>MEQAAPRVVAFLSDVGTHDEATGLCKGLMSRICPGVTIIDITHQVPAFDVVEGALMLEDVPEFFPEHTVICAYVYPETGSGTPTVAVRNDKGQLLVAPDNGLLTRALDASGVAEARLVTNPAVMNHPPTPTWYGRDVVAACAAHLAAGTPLADVGPVVDDPVRLPDVPFTRHESGLVGRVARIDRAFGNVWTNIPSAALGLPSTPDGPVTLDATVGGE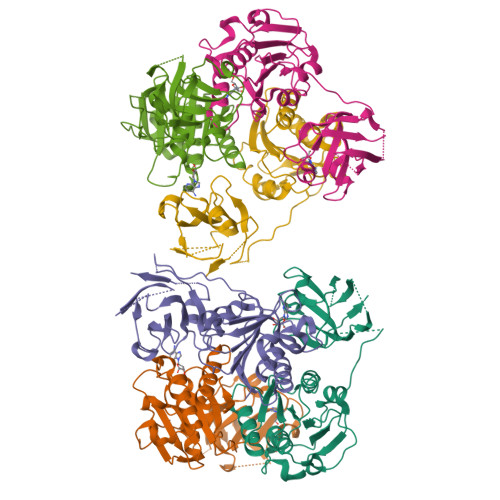RARWPWCTTFSQVATTGRLAYANSRGRLSFALNRGSLVAELGVAPDAPVEVHLPRVPG[6x]> METGNKYIEKRAIDLSRERDPNFFDNPGIPVPECFWFM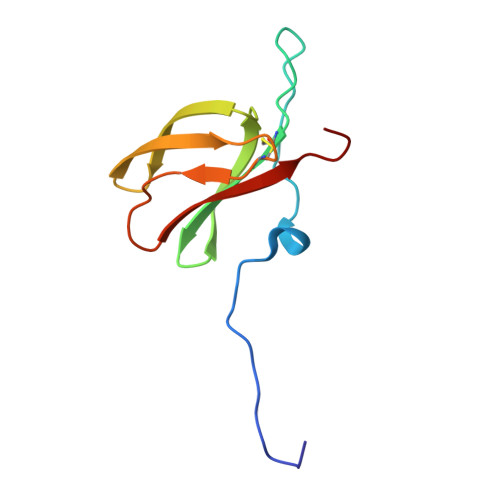FKNNVRQDAGTCYSSWKMDMKVGPNWVHIKSDDNCNLSGDFPPGWIVLGKKRPGF> MIIK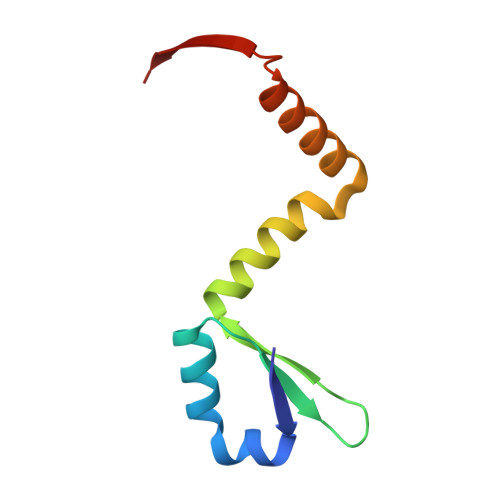NYSYARQNLKALMTKVNDDSDMVTVTSTDDKNVVIMSESDYNSMMETLYLQQNPNNAEHLAQSIADLERGKTITKDIDV> GAMAKTLDKKRIEQIKSECLRIYRIGIGHPSNSEILKYATEEEKKILIPILRKKPVRTISGVAVVAVMTSPAKCPHGKCIFCPGGLDSVFGDVPQSYTGREPATMRGLMFNFDPYLQTRARIEQLEKVGHPTDKIELIIMGGTFPAREIEYQDWFIKRCLDAMNERESKSLEEAQKINETAKHRCVALCIETRPDYCSEKEINQMLKLGATRVELGVQSIYNEILKLCKRGHSVEDTIKATQLLKDSGLKVSYHLMPGMPGSSIEMDKKMFKEIFTNPDFMPDMVKIYPCLVIEGTELYEMWKRGEFKPYREEEAIEVISYAKSIMPKWVRTSRIQRDIPATVIVDGVKKSNLGELVYKYMEKKGLRCRCIRCREVGHVYYKKGILPDPEHIKLVREDYEASGGTEIFLSFEDVKNDILIAFLRLRDPYKPFRKEIDDKTMLV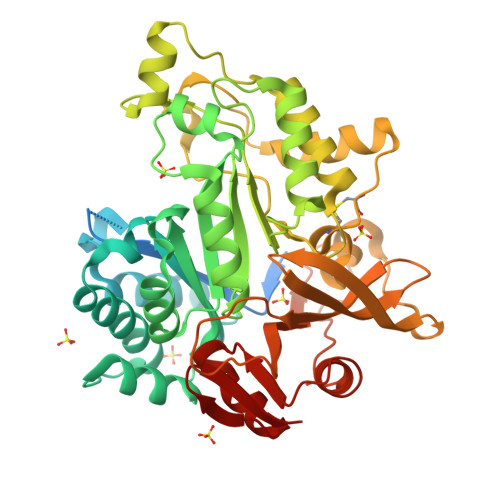RQLHVFGWEKALTRDIKEVSWQHMGYGRMLMKEAERIAKEEFGKKKILVTSGIGVREYYRKLGYKRVGAYMGKEL>GMSRKKNPSVIQFEKAITEKNYEAACTELLDILNKIDTNFGDIEGIDFDYPQQLETLMQDRIVYFCTRMSNAITQLFCDPQFSLSESGANRFFVVQRWLNLIFASSPYINADHILQTYNCNPERDSIYDIYLEPNKNVLMKFAVLYLPESNVNLNLDTMWETDKNICGSLCFALQSPRFIGTPAAFSKRSTILQWFPAKLEQFHVLDDLPSNISHDVYMHCSYDTAENKHNVKKALNQVIRSHLLKCGWQDRQITQIGMRNGKPVMVVVLEHFHSSHSIYRTHSTSMIAAREQFYLIGLGNNAVDQAGRDVFDEFHEFDGSNILKKLAFLKEMCEKNDAAVLYMPSIGMDLATIFVSNARFAPIQVIALGHPATTHSEFIEYVIVEDDYVGSESCFSETLLRLPKDALPYVPSSLAPTDVQYVLRETPEVVNIGIAATTMKLNPYFLETLKTIRDRAKVKVHFHFALGQSIGITHPYVARFIRSYLGDDATAHPHSPYNRYLDILHNCDMML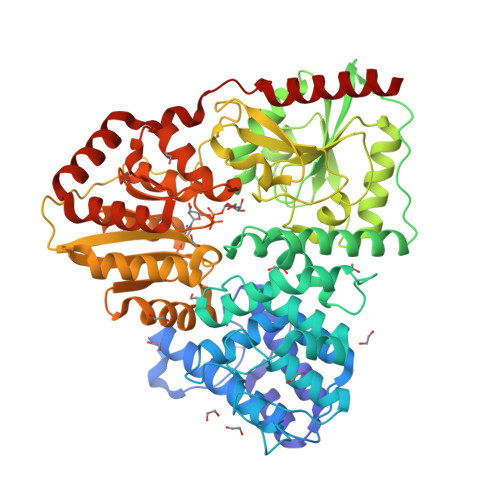NPFPFGNTNGIIDMVTLGLVGVCKTGPEVHEHIDEGLFKRLGLPEWLIADSVEDYIERAIRLAENHQERLALRRHIIENNGLKTLFSGDPSPMGKTLFAKLTEWRQTNGI[2x]>MRGNIRVYCRIRPALKNLENSDTSLINVNEFDDNSGVQSMEVTKIQNTAQVHEFKFDKIFDQQDTNVDVFKEVGQLVQSSLDGYNVCIFAYGQTGSGKTFTMLNPGDGIIPSTISHIFNWINKLKTKGWDYKVNCEFIEIYNENIVDLLRSDNNNKEDTSIGLKHEIRHDQETKTTTITNVTSCKLESEEMVEIILKKANKLRSTASTASNEHSSRSHSIFIIHLSGSNAKTGAHSYGTLNLVDLAGSARINVSQVVGDRLRETQNINKSLSCLGDVIHALGQPDSTKRHIPFRNSKLTYLLQYSLTGDSKTLMFVNISPSSSH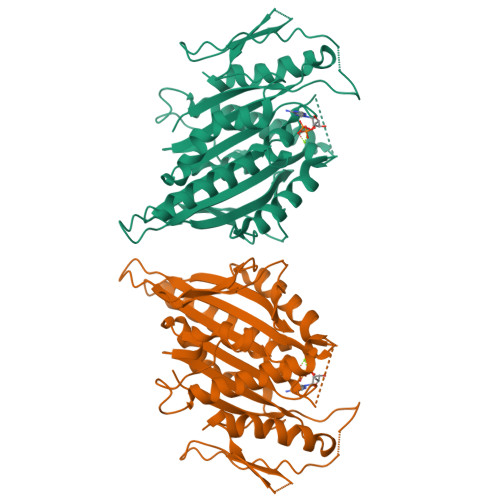INETLNSLRFASKVNSTRLVSRK[2x]> MEQQPLTLTAATTRAQELRKQLNQYSHEYYVKDQPSVEDYVYDRLYKELVDIETEFPDLITPDSPTQRVGGKVLSGFEKAPHDIPMYSLNDGFSKEDIFAFDERVRKAIGKPVAYCCELKIDGLAISLRYENGVFVRGATRGDGTVGENITENLRTVRSVPMRLTEPISVEVRGECYMPKQSFVALNEEREENGQDIFANPRNAAAGSLRQLDTKIVAKRNLNTFLYTVADFGPMKAKTQFEALEELSAIGFRTNPERQLCQSIDEVWAYIEEYHEKRSTLPYEIDGIVIKVNEFALQDELGFTVKAPRWAIAYKFPPEEAETVLEHHHH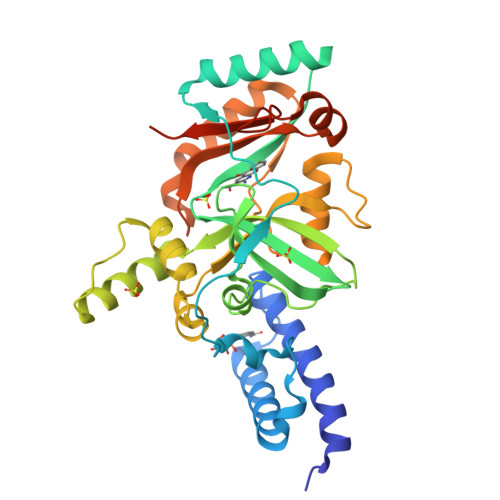HH butyl 3,4,5-tris(oxidanyl)benzoate | C11 H14 O5 | 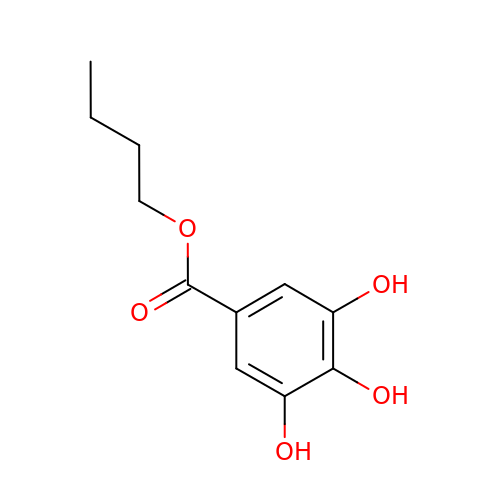XOPOEBVTQYAOSV-UHFFFAOYSA-N>GPSLRGLGARDHQATVVDKEYIAPHFVRVRLVSPTLFDEVIVEPTSWLRFWFPDPDGSDTEFQRAYTITESDPETGRFAVDMVLHEPAGPASTWARTVEPGATIAVMSMGSRGFSVPEDPEDRPVGYLLIGDSASTPAINGIIEVVPHDIPIELYLEQHHDDDVLIPLAEHPRLRVHRVSRDDASSL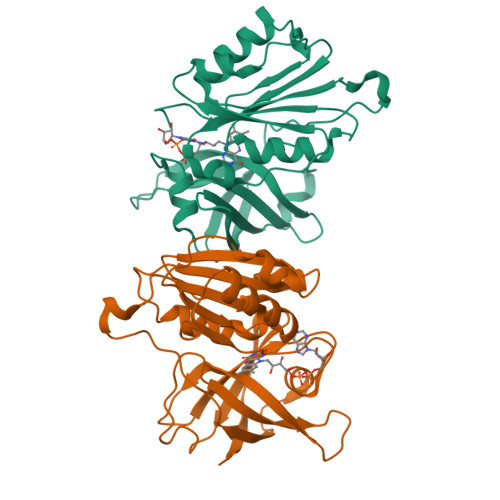AAALELRDWSNWYCWAGPEAGALKQVRTRLRDEFGFPKREVYAQAYWTEGRAMGSSRGETSTA[2x]> GCPQEDSDIAFLIDGSGSI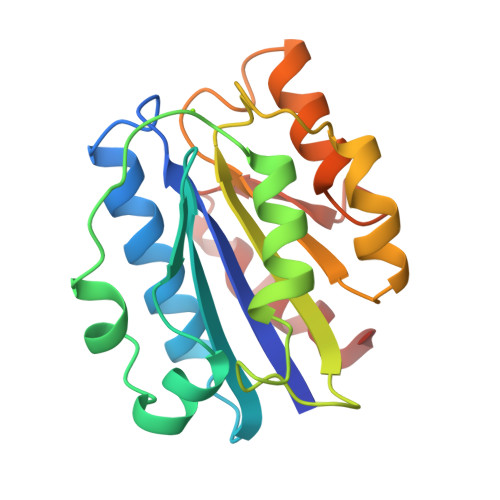IPHDFRRMKEFVSTVMEQLKKSKTLFSLMQYSEEFRIHFTFKEFQNNPNPRSLVKPITQLLGRTHTATGIRKVVRELFNITNGARKNAFKILVVITDGEKFGDPLGYEDVIPEADREGVIRYVIGVGDAFRSEKSRQELNTIASKPPRDHVFQVNNFEALKTIQNQLREK> MELMMAIGYLGLALVLGSLVAKIAEKLKIPDIPLLLLLGLIIGPFLQIIPSDSAMEIFEYAG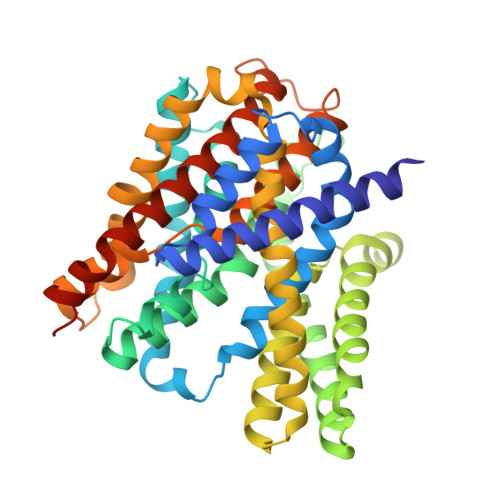PIGLIFILLGGAFTMRISLLKRVIKTVVRLDTITFLITLLISGFIFNMVLNLPYTSPVGYLFGAITAATDPATLIPVFSRVRTNPEVAITLEAESIFNDPLGIVSTSVILGLFGLFSSSNPLIDLITLAGGAIVVGLLLAKIYEKIIIHCDFHEYVAPLVLGGAMLLLYVGDDLLPSICGYGFSGYMAVAIMGLYLGDALFRADDIDYKYIVSFCDDLSLLARVFIFVFLGACIKLSMLENYFIPGLLVALGSIFLARPLGVFLGLIGSKHSFKEKLYFALEGPRGVVPAALAVTVGIEILKNADKIPASITKYITPTDIAGTIIIGTFMTILLSVILEASWAGMLALKLLGEYKPKYKEESHH> MGSSHHHHHHSSGHMNRQVIEFSKYNPSGNMTILVHSKHDASEYASIANQLMAATHVCCEQVGFIESTQNDDGNDFHLVMSGNEF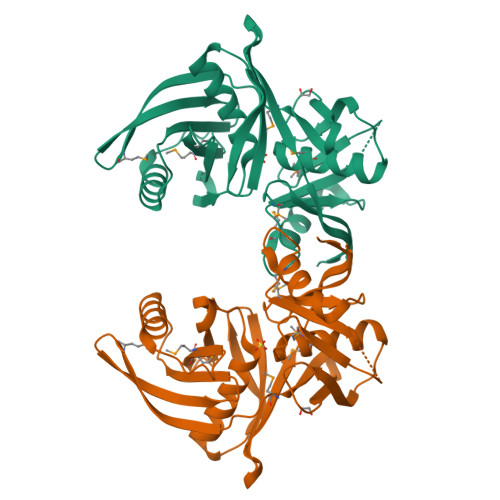SGNATMSYIHHLQESHLLKDQQFKVKVSGCSDLVQCAIHDCQYYEVQMPQAHRVVPTTINMGNHSWKALEIIYETYVHYVIPVKQVTTEIQHLVEAFVREQQWSHKYKTVGMMLFDEQRQFLQPLIYIPEIQSLIWENSCGSGTASIGVFNNYQRNDACKDFTVHQPGGSILVTSKRCHQLGYQTSIKGQVTTVATGKAYIE>[4x]HHHHHHSSGLVPRGSHMASMSKVGINGFGRIGRLVLRRLLEVKSNIDVVAINDLTSPKILAYLLKHDSNYGPFPWSVDFTEDSLIVDGKSIAVYAEKEAKNIPWKAKGAEIIVECTGFYTSAEKSQAHLDAGAKKVLISAPAGEMKTIVYNVNDDTLDGNDTIVSVASCTTNCLAPMAKALHDSFGIEVGTMTTIAAYTGTQSLVDGPRGKDLRASRAAAENI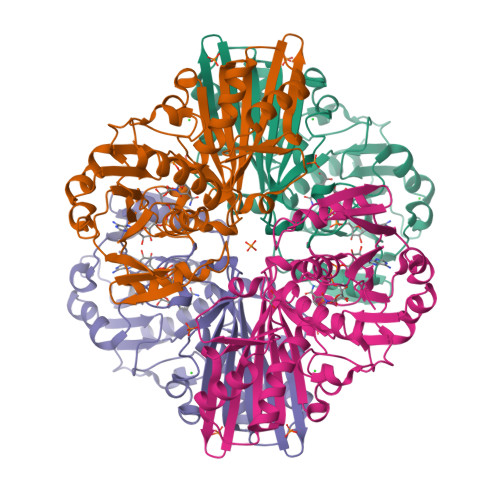IPHTTGAAKAIGLVIPELSGKLKGHAQRVPVKTGSVTELVSILGKKVTAEEVNNALKQATTNNESFGYTDEEIVSSDIIGSHFGSVFDATQTEITAVGDLQLVKTVAWYDNEYGFVTQLIRTLEKFAKL>[2x]VGTNTGGVLVITDTIIVKSGQTYDGKGIKIIAQGMGDGSQSENQKPIFKLEKGANLKNVIIGAPG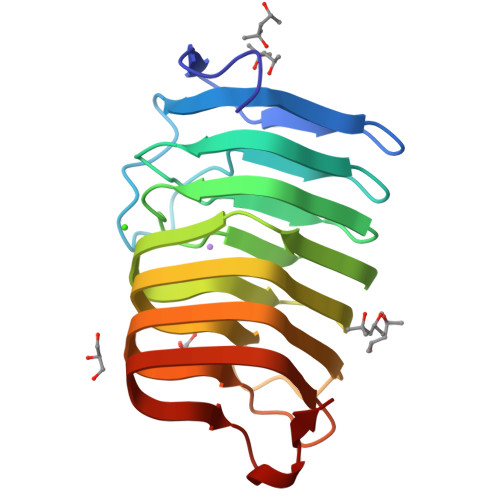CDGIHCYGDNVVENVVWEDVGEDALTVKSEGVVEVIGGSAKEAADKVFQLNAPCTFKVKNFTATNIGKLVRQNGNTTFKVVIYLEDVTLNNVKSCVAKSDSPVSELWYHNLNVNNCKTLFEFPSQSQIHQY>MILVFLGPPGAGKGTQAKRLAKEKGFVHISTGDILREAVQKGTPLGKKAKEYMERGELVPDDLIIALIEEVFPKHGNVIFDGFPRTVKQAEALDEMLEKKGLKVDHVLLFEVPDEVVIERLSGRRINPETGE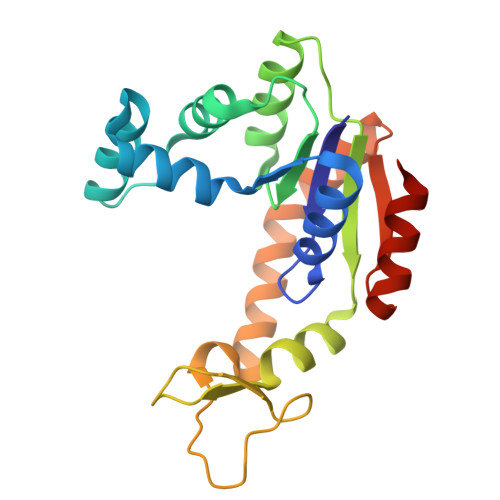VYHVKYNPPPPGVKVIQREDDKPEVIKKRLEVYREQTAPLIEYYKKKGILRIIDASKPVEEVYRQVLEVIGDGN[3x]> ETGSAQQLNEDLRLHL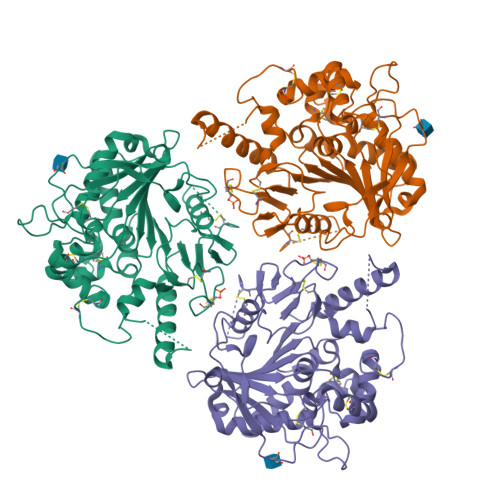LLNTSVTCNDGSPAGYYLKESRGSRRWLLFLEGGWYCFNRENCDSRYDTMSSLMSSRDWPRTRTGTGILSSQPEENPYWWNANMVFIPYCSSDVWSGASSKSEKNEYAFMGALIIQEVVRELLGRGLSGAKVLLLAGSSAGGTGVLLNVDRVAEQLEKLGYPAIQVRGLADSGWFLDNKQYRHTDCVDTITCAPTEAIRRGIRYWNGVVPERCRRQFQEGEEWNCFFGYKVYPTLRSPVFVVQWLFDEAQLTVDNVHLTGQPVQEGLRLYIQNLGRELRHTLKDVPASFAPACLSHEIIIRSHWTDVQVKGTSLPRALHCWDRSLHDSHKASKTPLKGCPVHLVDSCPWPHCNPSCPTGTKHHHHHH4-[(3,4-dimethoxyphenyl)methyl]morpholine 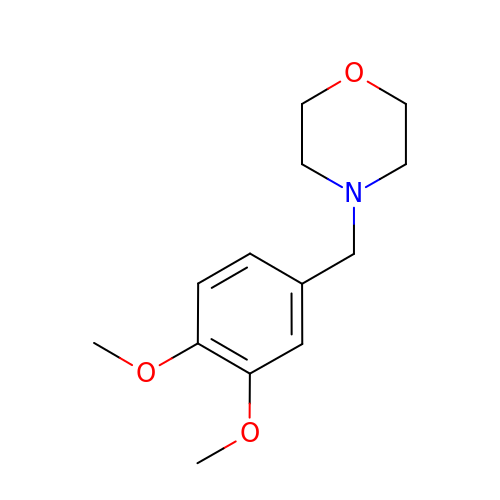| C13 H19 N O3 | BVODXXKHVBGLJY-UHFFFAOYSA-N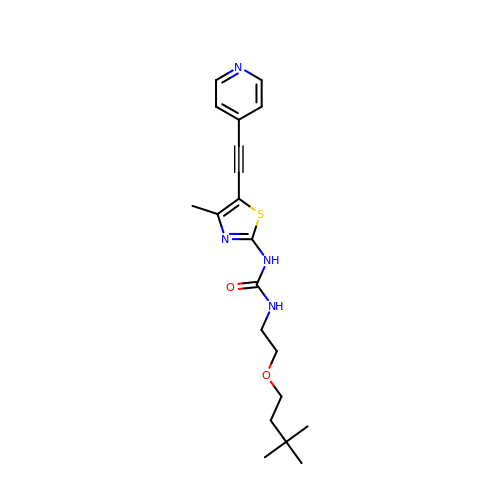N-[2-(3,3-dimethylbutoxy)ethyl]-N'-{4-methyl-5-[(pyridin-4-yl)ethynyl]-1,3-thiazol-2-yl}urea | C20 H26 N4 O2 S | LLAXZOBGRHVCCF-UHFFFAOYSA-N> AEGDDPAKAAFNSLQASATEYIGYAWAMVVVIV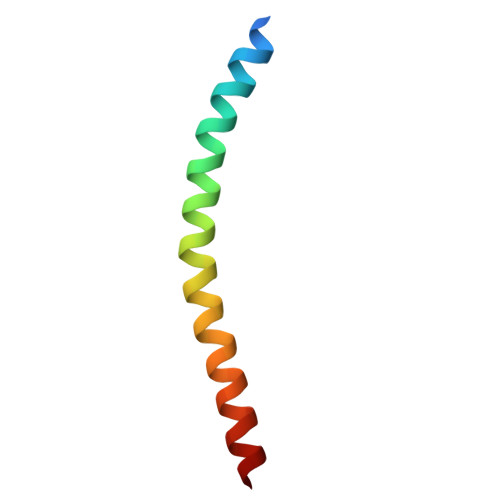GATIGIKLFKKFTSKAS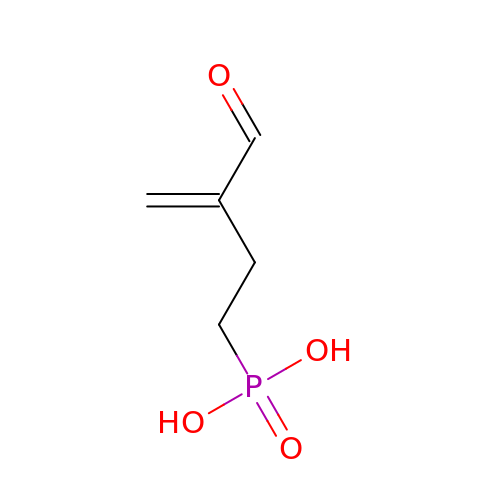(3-FORMYL-BUT-3-ENYL)-PHOSPHONIC ACID | C5 H9 O4 P | UBLMBCUBDKMVMQ-UHFFFAOYSA-N> MDHHHHHHHHASENLYFQGHMPNPVRFVYRVDLRSPEEIFEHGFSTLGDVRNFFEHILSTNFGRSYFISTSETPTAAIRFFGSWLREYVPEHPRRAYLYEIRADQHFYNARATGENLLDLMRQRQVVFDSGDREMAQMGIRALRTSFAYQREWFTDGPIAAANVRSAWLVDAVPVEPGHAHHPAGRVVETTRINEPEMHNPHYQELQTQANDQPWLPTPGIATPVHLSIPQAASVADVSEGTSAS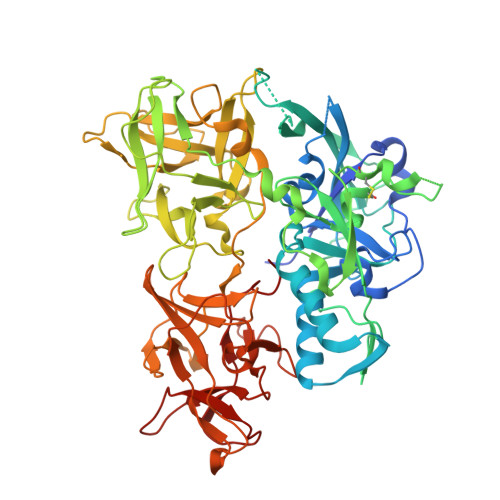LSFACPDWSPPSSNGENPLDKCIAEKIDNYNLQSLPQYASSVKELEDTPVYLRGIKTQKTFMLQADPQNNNVFLVEVNPKQKSSFPQTIFFWDVYQRICLKDLTGAQISLSLTAFTTQYAGQLKVHLSVSAVNAVNQKWKMTPQDIAITQFRVSSELLGQTENGLFWNTKSGGSQHDLYVCPLKNPPSDLEELQIIVDECTTHAQFVTMRAASTFFVDVQLGWYWRGYYYTPQLSGWSYQMKTPDGQIFYDLKTSKIFFVQDNQNVFFLHNKLNKQTGYSWDWVEWLKHDMNEDKDENFKWYFSRDDLTIPSVEGLNFRHIRCYADNQQLKVIISGSRWGGWYSTYDKVESNVEDKILVKDGFDRF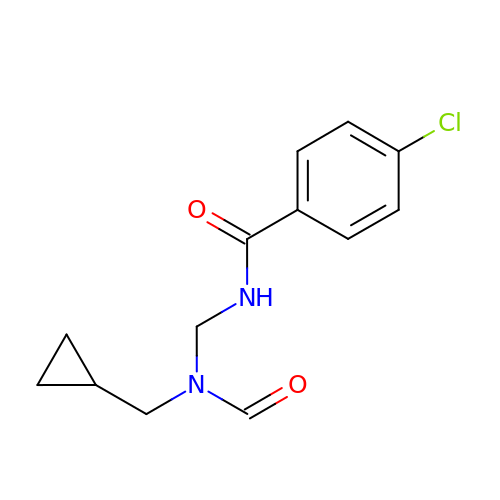4-chloranyl-N-[[cyclopropylmethyl(methanoyl)amino]methyl]benzamide | C13 H15 Cl N2 O2 | ZKBKHQJPIDEDKI-UHFFFAOYSA-N>[6x]MPAIFTHEGKVEGVPGNYPLTAENLFRIGLALCTLWILDKEIEEPTLSIPETNFVTLALSVGFMNAGGSVNVGKGGDIKLFLQKGEIYVLEFQPLSETDIKKLESILFGR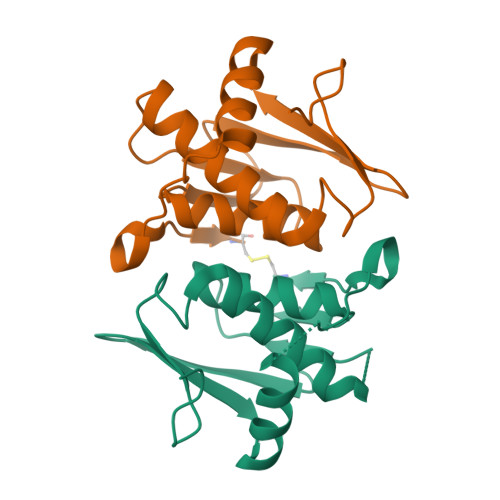APIPKKTGEDIGSFKC> MGSALFLVIFAYLLGSITFGEVIAKLKGVDLRNVGSGNVGATNVTRALGKKYGVLVFF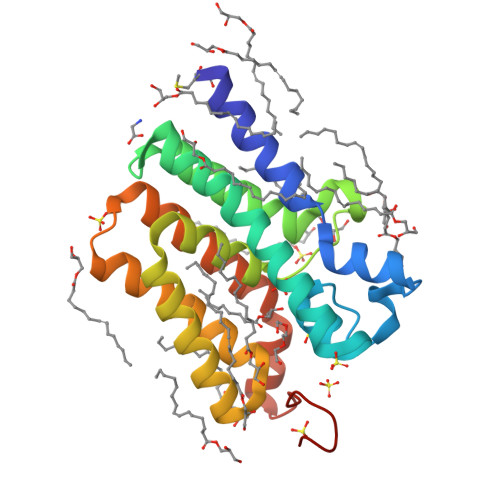LDFLKGFIPALIAVKSFGIDSWVLTFTGLASVLGHMYPVFFGFKGGKGVATALGVVFAVSPSVALFSFLVWLGIFLWKRYVSLASITATISAFLFLFVAGYPVNVLFMAIVIGALIIYRHRENINRLLTGREHRFGTLEVLFQ>[3x]MRGSHHHHHHGSGSGSGIEGRPYNGTGSRFNSSGAIAFGIQTLWTPPTSNPNCTVYTESDSLLSLCLTKC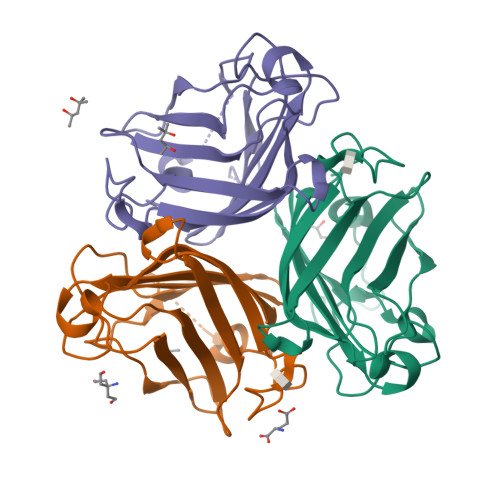GAHVLGSVSLTGVAGTMTNMAETSLAIEFTFDDTGKLLHSPLVNNTFSIRQGDSPASNPTYNALAFMPNSTLYARGGSGEPRNNYYVQTYLRGNVQRPITLTVTFNSAATGYSLSFKWTAVVREKFAAPATSFCYITEQ> MHHHHHHGAQPARSANDTVVVGSIIFTEGIIVANMVAEMIEAHTDLKVVRKLNLGGVNVNFEAIKRGGANNGIDIYVEYTGHGLVDILGFPATTDPEGAYETVKKEYKRK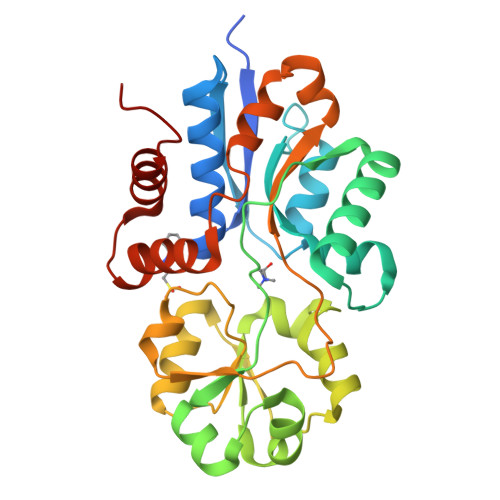WNIVWLKPLGFNNTYTLTVKDELAKQYNLKTFSDLAKISDKLILGATMFFLEGPDGYPGLQKLYNFKFKHTKSMDMGIRYTAIDNNEVQVIDAWATDGLLVSHKLKILEDDKAFFPPYYAAPIIRQDVLDKHPELKDVLNKLANQISLEEMQKLNYKVDGEGQDPAKVAKEFLKEKGLILQVD>[2x]MTRRIRIGGAQMGAISRSDSKKEIVDRLIALLRQASEKGCELVVF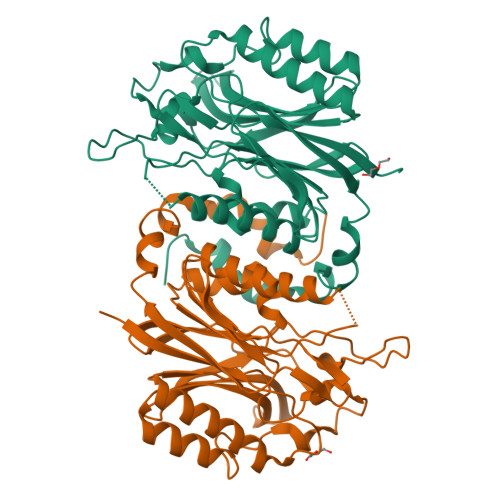PELALSTFFPRWYAERDGMDGYFEDGMPNAATLPLFEEARRLGIGFSLGYAELVQEDGRVRRFNTTVLVERNGEIVGKYRKIHLPGHAEYEPERSHQHLEKRYFEVGNTGFQVWDAFGGRVGMAICNDRRWVETYRVMGLQNVELILIGYNTPVNDSLSGESETLGMFHNHLTMQAGAYQNSTWVVGVAKAGVEDGHRLMGGSVIVAPTGEIVAQAMTEGDELIVADCDLDRCRYYKSHIFNFAAHRRPEFYQRITSQTGVE>[3x]GPGSMRRRRAAHRRFLPRPRPLNARRNAPIHSSSTSSIATNMSQQLQQIIDNAWENRAELSPKAASAEIREAVAHAIEQLDRGALRVAEKIDGAWTVHQWLKKAVLLSFRLEDNAPMPAGGYSQFYDKVPSKFANYTAEDFAAGGFRVVPPAIARRGSFIAKNVVL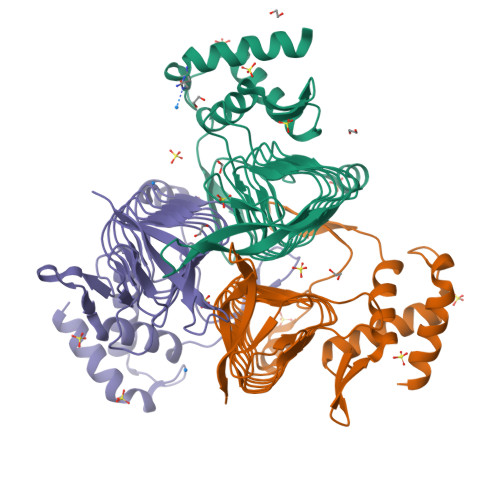MPSYTNIGAYVDEGTMVDTWATVGSCAQIGKNVHLSGGVGIGGVLEPLQANPVIIEDNCFIGARSEVVEGVIVEENSVISMGVYLGQSTKIYDRETGEVTYGRIPAGSVVVAGNLPAKDGTHSLYCAVIVKKVDAKTRAKVGLNELLRGD>[2x]MTTKPFFDAARVIAGGKLTQAQVDELNKVVNKLAPGGKTTSDVGVNLISGFEGTRFTAYDDGVGIWTIGTGTTVYPNGVKVKKGDTCTPEQAKSYFKHDLAKFEKTVNESVTVPLTQNQFDALVSLTYNIGAGALKNSTLLKLLNKGDYKGAADQFLVWNKAGGKVLKGLVRRREAERALFLKK

As a proof-of-concept, five peptidoglycan hydrolases from the Acinetobacter baumannii proteome (PHAb7-PHAb11) were identified using PlyF307 lysin-derived peptide as a template. To understand the catalytic mechanism and thermal stability of these peptidoglycan hydrolases, we attempted to decipher their structures and eventually obtained the crystal structures of PHAb8, PHAb10, and PHAb11 by X-ray crystallography. Despite their lower amino acid sequence similarity, PHAb8, PHAb10, and PHAb11 superimposed well with T4 lysozyme, especially in their Glu-Asp-Thr catalytic triad regions, suggesting that PHAb8, PHAb10, and PHAb11 may be phage-originated. All these observations together indicated that PHAb8, PHAb10, and PHAb11 were highly evolutionarily related to T4 lysozyme and might share similar catalytic mechanisms of action.

Structural prediction analysis showed that PHAb10 contains a putative lysozyme catalytic domain (amino acids 1–110, P10-Lys) and a C-terminal cationic peptide (amino acids 111–149, P10-CP), whereas PHAb11 contains an N-terminal cationic peptide with unknown function (amino acids 1–36, P11-NP), followed by a putative lysozyme catalytic domain (amino acids 37–145, P11-Lys, with 68.5% sequence similarity with P10-Lys) and a C-terminal cationic peptide (amino acids 146–184, P11-CP, which shows 94.9% sequence similarity with P10-CP). Results showed that PHAb8 was a monomer, while PHAb10 and PHAb11 formed an asymmetric dimer. The two subunits of PHAb11 formed a tail-to-tail dimer with a rotation angle of –179.4° along the rotation axis and a distance of 37.1 Å between them. Each PHAb11 monomer contained an independent substrate-binding cavity around its catalytic triad. Notably, the N-terminal 36 amino acids, P11-NP, were missing in our PHAb11 dimer. We speculated that it may be destroyed during crystal formation. Structure-based homology analysis revealed that PHAb10 and PHAb11 probably belonged to the T4 lysozyme family and possessed the conserved Glu-Asp-Thr catalytic triad shared by traditional phage lysins and bacterial autolysins, namely Glu17, Asp26, and Thr32 of PHAb10, and Glu52, Asp61, and Thr67 of PHAb11. Our results showed that PHAb8, PHAb10, and PHAb11 were denatured with transition temperatures of 41.4°C, 53.7°C, and 59.9°C, respectively. Interestingly, signs of aggregation were only observed in PHAb8 but not in PHAb10 and PHAb11, indicating that PHAb10 and PHAb11 underwent structural refolding without precipitation during heat treatment. Similar to the folding-refolding phenomenon of PHAb10, PHAb11 and its N-terminal peptide-deleted variant P11-C could restore to their native conformation after 1 hr treatment at 100°C, while its C-terminal peptide-deleted variant P11-N could not refold to its native conformation, indicating that C-terminal peptide was essential for its hyper-thermostability.> MGHHHHHHGDAALLLNVEGVKKTILHGGTGELPNFITGSRVIFHFRTMKCDEERTVIDDSRQVGQPMHIIIGNMFKLEFWEILLTSMRVHEVAEFWCDTIHTGVYPILSRSLRQMAQGKDPTEWHVHTC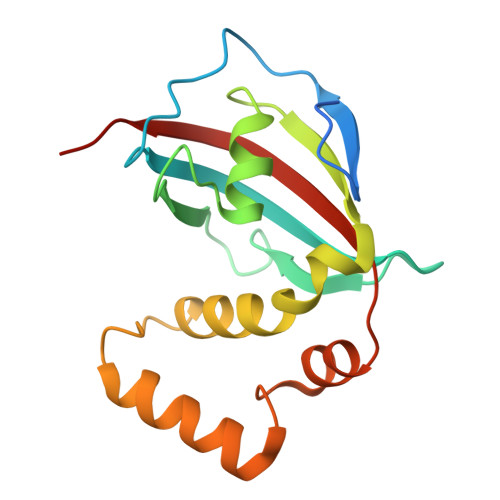GLANMFAYHTLGYEDLDELQKEPQPLVFVIELLQVDAPSD>[4x]METERKSRICVTGA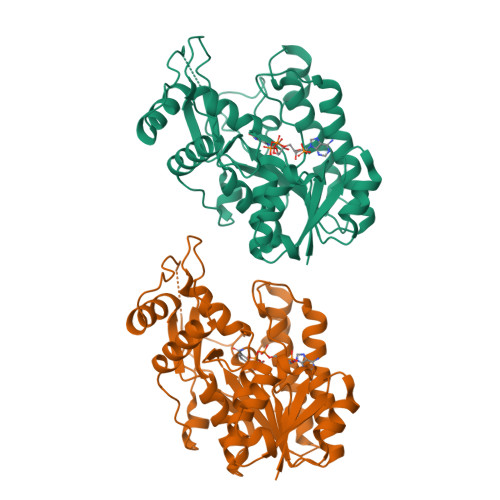GGFVASWVVKLFLSKGYLVHGTVRDLGEEKTAHLRKLEGAYHNLQLFKADLLDYESLLGAITGCDGVLHVATPVPSSKTAYSGTELVKTAVNGTLNVLRACTEAKVKKVIYVSSTAAVLVNPNLPKDKIPDEDCWTDEEYCRTTPFFLNWYCIAKTAAEKNALEYGDKEGINVISICPSYIFGPMLQPTINSSNLELLRLMKGDDESIENKFLLMVDVRDVAEAILLLYEKQETSGRYISSPHGMRQSNLVEKLESLQPGYNYHKNFVDIKPSWTMISSEKLKKLGWKPRPLEDTISETVLCFEEHGLLENE> LKESPSGYLRSGEGDTGCGELVWVGEPLTLRTAETITGKYGV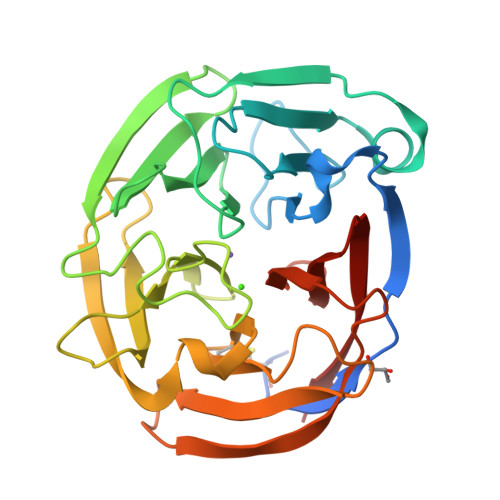WMRDPKPTYPYTQETTWRIDTVGTDVRQVFEYDLISQFMQGYPSKVHILPRPLESTGAVVYSGSLYFQGAESRTVIRYELNTETVKAEKEIPGAGYHGQFPYSWGGYTDIDLAVDEAGLWVIYSTDEAKGAIVLSKLNPENLELEQTWETNIRKQSVANAFIICGTLYTVSSYTSADATVNFAYDTGTGISKTLTIPFKNRYKYSSMIDYNPLEKKLFAWDNLNMVTYDIRLSKM>[4x]MSLNKNLVAQRFAKAGQSYSKHAIVQKQICQNLTNLLKQFCPSAMSRVFEIGCGSGNLTRLLVESFQIENLVLNDLYAEVQQHFNHEEHVKWLIGDVETLEFPQQLD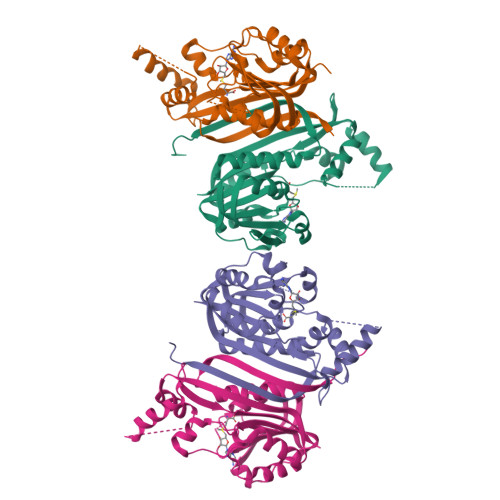MIVSGSALQWMQDLPRLLQHCYAALNEQGWLCFSTFGPKNLIEIKELTGQGLNYWNLENWNSALTQAGFEILHLAQSETQLYFDSPKAVLQHLKATGVTATAQHRWTKQSLQQFYQDYDRFKHTEGYSLTYHPIYCIARRMK> GASRASRSHSRREEHSGRNGLHHPSPDHFWPRFPDALRPFVPWDQLENEDSSVHISPRQKRDANSSIYKGKKCRMESCFDFTLCKKNGFKVYVYPQQKGEKIAESYQNILAAIEGSRFYTSDPSQACLFVLSLDTLDRDQLSPQYVHNLRSKVQSLHLWNNGRNHLIFNLYSGTWPDYTEDVGFDIGQAMLAKASISTENFRPNFDVSIPLFSKDHPRTGGERGFLKFNTIPPLRKYMLVFKGKRYLTGIGSDTRNALYHVHNGEDVVLLTTCKHGKDWQKHKDSRCDRDNTEYEKYDYREMLHNATFCLVPRGRRLGSFRFLEALQAACVPVMLSNGWELPFSEVINWNQAAVIGDERLLLQIPSTIRSIHQDKILALRQQTQFLWEAYFSSVEKIVLTTLEIIQDRIFKHISRNSLIWNKHPGGLFVLPQYSSYLGDFPYYYANLGLKPPSKFTAVIHAVTPLVSQSQPVLKLLVAAAKSQYCAQIIVLWNCDKPLPAKHRWPATAVPVVVIEGESKVMSSRFLPYDNIITDAVLSLDEDTVLSTTEVDFAFTVWQSFPERIVGYPARSHFWDNSKERWGYTSKWTNDYSMVLTGAAIYHKYYHYLYSHYLPASLKNMVDQLANCEDILMNFLVSAVTKLPPIKVTQKKQYKETMMGQTSRASRWADPDHFAQRQSCMNTFASWFGYMPLIHSQMRLDPVLFKDQVSILRKKYRDIERLNNNNNNGHHHHHHHH;> GASPHSIESSNDWNVEKRSIRDVPVVRLPADSPIPERGDLSCRMHTCFDVYRCGFNPKNKIKVYIYALKKYVDDFGVSVSNTISREYNELLMAISDSDYYTDDINRACLFVPSIDVLNQNTLRIKETAQAMAQLSRWDRGTNHLLFNMLPGGPPDYNTALDVPRDRALLAGGGFSTWTYRQGYDVSIPVYSPLSAEVDLPEKGPGPRQYFLLSSQVGLHPEYREDLEALQVKHGESVLVLDKCTNLSEGVLSVRKRCHKHQVFDYPQVLQEATFCVVLRGARLGQAVLSDVLQAGCVPVVIADSYILPFSEVLDWKRASVVVPEEKMSDVYSILQSIPQRQIEEMQRQARWFWEAYFQSIKAIALATLQIINDRIYPYAAISYEEWNDPPAVKWGSVSNPLFLPLIPPQSQGFTAIVLTYDRVESLFRVITEVSKVPSLSKLLVVWNNQNKNPPEDSLWPKIRVPLKVVRTAENKLSNRFFPYDEIETEAVLAIDDDIIMLTSDELQFGYEVWREFPDRLVGYPGRLHLWDHEMNKWKYESEWTNEVSMVLTGAAFYHKYFNYLYTYKMPGDIKNWVDAHMNCEDIAMNFLVANVTGKAVIKVTPRKKFKCPECTAIDGLSLDQTHMVERSECINKFASVFGTMPLKVVEHRADPVLYKDDFPEKLKSFPNIGSLNNNNNNGHHHHHHHH

Heparan sulfates are complex polysaccharides that mediate the interaction with a broad range of protein ligands at the cell surface. A key step in heparan sulfate biosynthesis is catalyzed by the bi-functional glycosyltransferases EXT1 and EXT2, which generate the glycan backbone consisting of repeating N-acetylglucosamine and glucuronic acid units. EXT1 and EXT2 are predicted to share a common architecture with a N-terminal transmembrane helix anchoring the enzymes in the Golgi membrane, followed by the glucuronic acid transferase (GlcA-T) domain and the C-terminal N-acetylglucosamine transferase (GlcNAc-T) domain. Here, we present the cryo-electron microscopy structure of human EXT1-EXT2, which reveals the formation of a tightly packed hetero-dimeric complex harboring four glycosyltransferase domains.

Single-particle cryo-EM studies on EXT1-EXT2, in presence of both UDP-sugar donor substrates and divalent manganese ions, provided a three-dimensional EM reconstruction with an overall resolution of 2.8 Å. We de novo built an almost complete model of EXT1-EXT2, only lacking the presumably flexible N-terminal stem regions (residues 29-88 in EXT1, residues 47-77 in EXT2) connecting the catalytic Golgi-luminal domain to the transmembrane anchoring helices, as well as several short, surface-exposed loops. EXT1 and EXT2 form a tightly packed 1:1 hetero-dimeric complex with a total interaction surface of 3523 Å2, suggesting that EXT1-EXT2 complex formation is essential for protein stability. The N-terminal glycosyltransferase domains of EXT1 (residues 89-435) and EXT2 (residues 78-419), supposedly harboring GlcA-T activity, adopt a characteristic GT-B fold architecture. The C-terminal glycosyltransferase domains, formed by residues 479-728 in EXT1 and residues 455-702 in EXT2, feature a GT-A fold and potentially harbour GlcNAc-T activity. The GlcA-T and GlcNAc-T domain of EXT1 interact tightly with each other, while the two domains of EXT2 are only connected through a potentially flexible hinge region. When analyzing the GlcA-T active site of EXT1, we found an additional EM density that fits a UDP ligand. The UDP is bound by several charged residues (Arg280, Arg346, Glu349), through a pi-stacking interaction with Tyr324 and a hydrogen bond with Tyr319. Surprisingly, the active site of the EXT2 GlcA-T domain displayed a different topology, with an anti-parallel beta-sheet intruding into the donor substrate binding pocket.> MAKQQNNRRKSATMRAV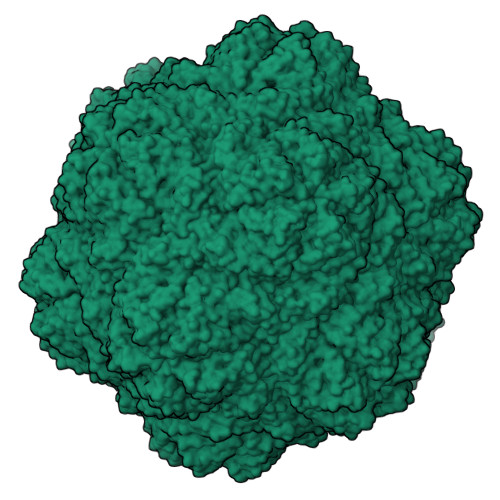KRMINTHLEHKRFALINSGNTNATAGTVQNLSNGIIQGDDINQRSGDQVRIVSHKLHVRGTAITVSQTFRFIWFRDNMNRGTTPTVLEVLNTANFMSQYNPITLQQKRFTILKDVTLNCSLTGESIKDRIINLPGQLVNYNGATAVAASNGPGAIFMLQIGDSLVGLWDSSYEAVYTDA>SNALEDSSTISFITWNIDGLDGCNLPERARGVCSCLALYSPDVVFLQEVIPPYCAYLKKRAASYTIITGNEEGYFTAI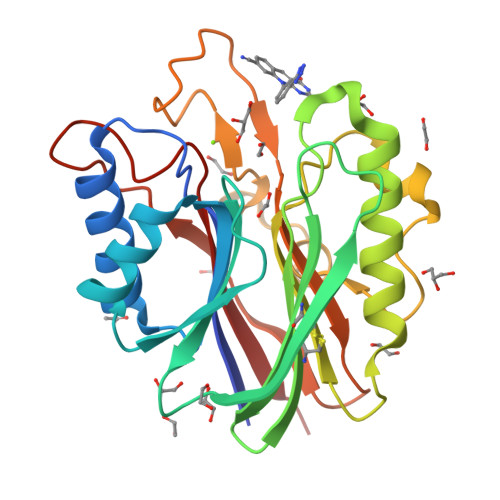LLKKGRVKFKSQEIIPFPNTKMMRNLLCVNVSLGGNEFCLMTSHLESTRGHSAERIRQLKTVLGKMQEAPDSTTVIFAGDTNLRDREVIKCGGLPDNVFDAWEFLGKPKHCQYTWDTKANNNLRIPAACKLRFDRIFFRAEEGHLIPQSLDLVGLEKLDCGRFPSDHWGLLCTLNVVL[2x]2-METHYLIMIDAZOLE | C4 H6 N2 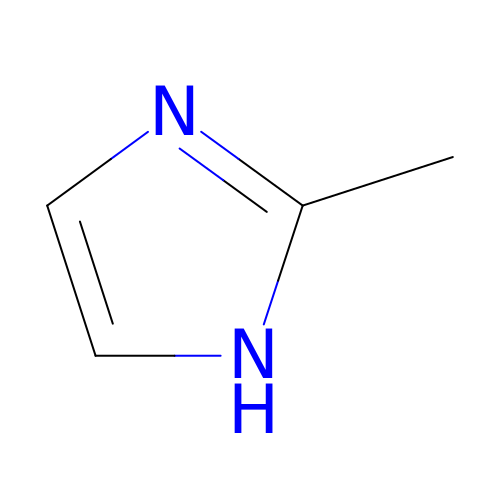| LXBGSDVWAMZHDD-UHFFFAOYSA-N> DSFSLLSQITPHQRCSFYAQVIKTWYSDKNFTLYVTDYTENELFFPMSPYTSSSRWRGPFGRFSIRCILWDEHDFY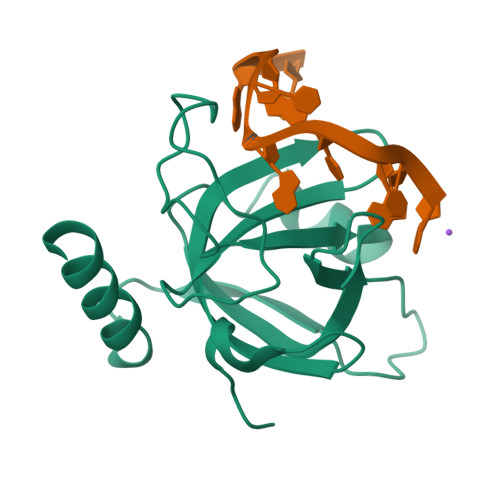CRNYIKEGDYVVMKNVRTKIDHLGYLECILHGDSAKRYNMSIEKVDSEEPELNEIKSRKRLYVQN Nonribosomal peptide synthetases (NRPSs) produce small peptides as secondary metabolites in fungi and bacteria. Tomaymycin is synthesized in Streptomyces and Micrococci by an NRPS consisting of the initiation module TomA and the elongation/termination module TomB. TomB contains a C domain (BC; TomB91–533), an A domain (BA; TomB534–1055), which functions to load the ppant arm of its PCP domain (BPCP; TomB1056–1141) with 4-ethylidene proline, and a reductase domain (BR; TomB1142–1535). The C domain binds two substrate-loaded PCPppant domains—termed the donor and acceptor PCPs—and transfers the growing peptide chain from the donor PCP of the upstream module onto the aminoacyl subunit carried by the acceptor PCP of the same module.

The crystallization construct comprised residues 1 to 533; however, the first 79 residues did not yield resolvable electron density, resulting in crystal structures of only the BC domain (91 to 533) and the preceding 11 amino acids. In neither form was there observable electron density for the first 79 residues. As other canonical C domains, TomB80–533 consists of N-terminal and C-terminal lobes, which adopt a chloramphenicol acetyltransferase fold and are arranged in a V shape. Two crossover elements extend from the C-terminal to the N-terminal lobe: the “floor” loop between β8 and β9 and the “latch” loop between β10 and β11. The catalytic tunnel is at the interface between the two lobes and includes the conserved motif 222HHXXXD227, where H223 is fundamental for catalysis. In both crystal forms, the catalytic tunnel of BC is wide enough to accommodate the ppant arm and their substrates at both the donor and acceptor sites. The tunnel is ~38 Å long with a minimum width of ~1.4 Å at the bottleneck, as measured by CAVER 3.0 (29).

>[2x]GPMLMNSPLRTTVLDLARTTLGSADLTAHEPLADRCEHPALLDDLATTLTAVFAVEITGADLAAGATVADVAARMDDRRDAPRIPELRAGLAPRDGRAVEASFGQSGIWLIDQYLPNPAAYNGPFFVRLPFSADPDRLHAAVRGVLRRQEVLRTTYALSDGTLRQNVSRDDDAVVFEVARYGDDKELDALVHRVANLRLDLARGPVIAVTCALGPANRSAVICNIHHIASDAASAGVFLRELLDAYDRLGRGLPVEADPLRPTYGDFSQWYRELMNPEALTRSLDHFAARLAGELPVLDLPTDRPRPPVKQHRGGTLPLHLPAAAADDFEALARTEGVTLFMALVAAYAVFLSRHTGQRRVLIGSPVSLRDDPATHELIGYFVNLVVLQQEIDDRMTVRDVLRRAREEVSEALRHKWAPFDKVVERLQPPRSSGYTPLVQTMLVLTQGDAGRISHDDTELRIERGAAHGAKYDLSLVFERDSEGLHGLIEYDADLFDEPTVRAMGDRLRHLMEQFARRPDAPLHELEALGAQERRSV>AGITGTWYNQLGSTFIVTAGADGALTGTYESAVGNAESRYVLTGRYDSAPATDGSGTALGWTVAWKNNYRNAHSATTWSGQYVGGAEARINTQWLLTSGTTEANAWKST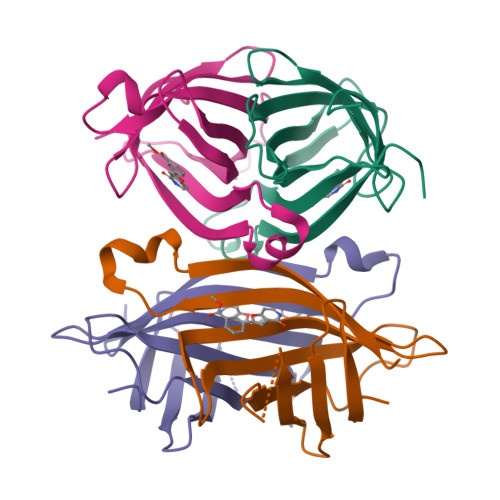LVGHDTFTKVKP[4x]>[9x]MDLTHFQDGRPRMVDVTEKPETFRTATAEAFVELTEEALSALEKGGVGKGDPLVVAQLAGILAAKKTADLIPLCHPLPLTGVEVRVELLKA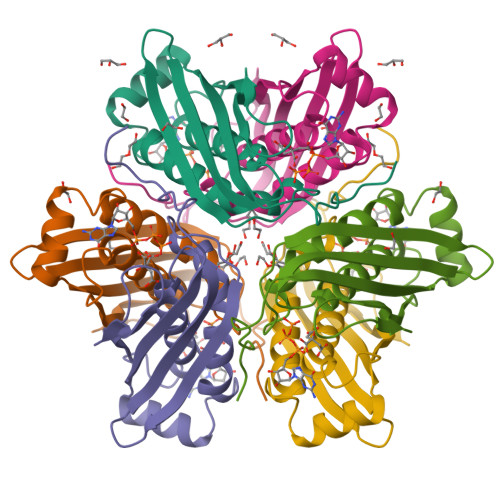EKRVRIEATVKTKAETGVEMEAMTACAVAALTVYDMLKAASKGLVISQVRLLHKAGGKSGEWRREQ Specifically, SV40 small t antigen (ST) binds to and perturbs the function of the abundant protein phosphatase 2A (PP2A). PP2A is a family of heterotrimeric enzymes, composed of a structural A subunit, a catalytic C subunit, and one of several regulatory B subunits. SV40 ST consists of an N-terminal J domain and a C-terminal unique domain that contains two separate zinc-binding motifs. SV40 ST binds to the same region of PP2A as the regulatory subunit B56, which provides a structural explanation for the displacement of regulatory B subunits by SV40 ST.

We have determined the crystal structure of full-length SV40 ST in complex with the full-length Aα subunit of PP2A. Crystal structure of the complex was determined by a combination of molecular replacement, using the PP2A A subunit structure as the searching model, and single-wavelength anomalous dispersion of intrinsic zinc atoms in ST, and was refined at 3.1 Å resolution. Four complexes were found in each asymmetric unit. In each complex, the scaffolding A subunit contains 15 HEAT repeats that forms a horseshoe shape. The four A-ST complexes in the asymmetric unit have essentially the same structure, except HEAT repeats 11–15 that show substantial conformational variation (see below). ST contains an N-terminal J domain and a C-terminal unique domain. These two domains sit on the concave and convex sides of the ridge of the A subunit horseshoe structure, respectively, by interacting with intra-repeat loops of the Aα subunit HEAT repeats 3–7, which is also the binding site for B56γ1 in the A-B56γ1-C trimeric PP2A holoenzyme structure. The first zinc-binding site is positioned between two roughly parallel helices (α4 and α5) and the L5 loop, coordinated by four conserved cysteine residues (Cys103, Cys111, Cys113, and Cys116). The second zinc is located between two roughly perpendicular helices (α5 and α6) and coordinated by three conserved cysteines in the second cysteine cluster (Cys138, Cys140, and Cys143), with Cys140 and Cys143 from the N-terminal end of α6 and the conserved His122 from the middle of α5. The position of the indole ring of Trp140 is flipped between these two complex structures, mostly due to the intercalation of Pro132 of ST between Trp140 and Phe141 by forming a hydrophobic core. The linker between helices 2 and 3, which has been implicated in Hsp70 interaction, as well as the linker between J and unique domains (residues 72–86), is not visible in any of the four complexes in the asymmetric unit, suggesting structural flexibility of these two linkers in the A-ST complex.

>[4x]MAAADGDDSLYPIAVLIDELRNEDVQLRLNSIKKLSTIALALGVERTRSELLPFLTDTIYDEDEVLLALAEQLGTFTTLVGGPEYVHCLLPPLESLATVEETVVRDKAVESLRAISHEHSPSDLEAHFVPLVKRLAGGDWFTSRTSACGLFSVCYPRVSSAVKAELRQYFRNLCSDDTPMVRRAAASKLGEFAKVLELDNVKSEIIPMFSNLASDEQDSVRLLAVEACVNIAQLLPQEDLEALVMPTLRQAAEDKSWRVRYMVADKFTELQKAVGPEITKTDLVPAFQNLMKDCEAEVRAAASHKVKEFCENLSADCRENVIMTQILPCIKELVSDANQHVKSALASVIMGLSPILGKDNTIEHLLPLFLAQLKDECPEVRLNIISNLDCVNEVIGIRQLSQSLLPAIVELAEDAKWRVRLAIIEYMPLLAGQLGVEFFDEKLNSLCMAWLVDHVYAIREAATSNLKKLVEKFGKEWAHATIIPKVLAMSGDPNYLHRMTTLFCINVLSEVCGQDITTKHMLPTVLRMAGDPVANVRFNVAKSLQKIGPILDNSTLQSEVKPILEKLTQDQDVDVKYFAQEALTVLSLA;>MDKVLNREESLQLMDLLGLERSAWGNIPLMRKAYLKKCKEFHPDKGGDEEKMKKMNTLYKKMEDGVKYAHQPDFGGFWDATEVFASSLNPGVDAIYCKQWPECVKKMSTNCICLLCLLRMKHENRKLYRKDPLVWVDCYCFDCFRMWFGLDLCEGTLLLWCDIIGQTTYRDLKL[4x]Psychrophilic β-d-galactosidase from Arthrobacter sp. 32cB is an interesting candidate for industrial use, as it can hydrolyze lactose at rate comparable to mesophilic βDG from Kluyveromyces lactis. Furthermore, it exhibits additional transglycosylation activity, it catalyzes synthesis of GOS and HOS, for example: lactulose and alkyl glycosides. The functional dimer of ArthβDG has two independent active sites. Each of them is located on the top of TIM-barrel Domain 3 and is constituted of residues from both subunits of the dimer.

The question of the effect of point mutation of the other catalytic residue, E517, has not been answered before. The ArthβDG_E517Q exhibited no catalytic activity, whereas activity of mutant ArthβDG_D207A was severely depleted. As expected of the mutation of the catalytic residue, E517 into glutamine caused loss of function of the enzyme. Mutation of catalytic residue E517 into glutamine resulted in the elevation of the melting temperature of the mutant in respect to ArthβDG by 3.5–5 °C, depending on the investigated buffer solution. In the case of 50 mM sodium phosphate pH 6.0, it attained 49 °C, which means that it was higher by 4.5 °C compared to wild-type protein. The structures of ArthβDG mutants: ArthβDG_D207A and ArthβDG_E517Q, were solved proving that the point mutations within the active site of ArthβDG have no destabilizing effect on protein’s structure. In the case of ArthβDG_E517Q, only a slight change in character of the active site was observed —similar to previously studied loss of function mutant ArthβDG_E441Q. The inactive mutant E517Q was designed specially to enable binding of transglycosylation product—lactulose, in the active site of enzyme and thus elucidating the mode of its binding.

> MSVETPSALADSSPHTAPGSAGRSLELGAADIQDLESFEAGRGALPARAYLQSDAPRLSLNGEWQFRLSPGSRVAPDDGWQLGEALNGFESLPVPSSWPMHGHGAPAYTNVQFPFAVEPPHVPEANPIGDHLVVFEAGPEFFPHALLRFDGIESAGTVWLNGVELGTTRGSRLAHEFDVSGILEQGENTLAVRVAQFSAASYVEDQDMWWLPGIFRDVTLQARPAAGIDDVFVHAGYDHITGEGILKVEASRGGQAIDAVVRVPELALELAAGTEVRVPAVEPWSAEVPKLYEAAVSAAGESVALQIGFRSIAIEDAQFKVNGRRILLRGVNRHEHHPRLGRVVPRDVVEAELRLMKQHNINAIRTSHYPPHPQFLALADQLGFYVVLECDLETHGFESAGWAQNPSDDPQWEDALVDRMRRTVERDKNHASVVMWSLGNEAGTGRNLAAMSRWTKDRDPSRPIHYEGDWSSEHVDVYSRMYASQAETALIGQGIEPALNDAALDARRRAMPFVLCQYVHAMGNGPGGMSEYQALFEKYPRLMGGFVWEWLEHGITVSTADGVDHYGYGGDFGEEVHDGNFVTDGLVDADRRPRPGLLDFKKVIEPLRIDVARDWTGFTLRNGQDFADTSAFSFRYEVEADGGALDGGTVDVAPVAPQSETVVELPGSVAALAAGLSDGRPAVLTVRAVLGADSAWADAGHEVAWGQSVREPGAPVPPAPVEPVQVQDSELTLGPVVFSRATGMPTSIGGVPVEKLGLTLWWAPTDNDLGREWGGADERPLATQWKDAGLNRLHTRLLGISANPGQDGGETLTVRTRVSAADKQYGVLVDYTWSTDGETVGLRTQVRRDGTWVNRGFEVEWARIGLEFVLGEETELVSWFGQGPHQSYPDTGQGARAGWFSLPLAKMDVEYVRPQECGARSGSRSAALQLGGRTLEICGDPFALTVRPYSQDVLDAAAHRPDLKADGRTYLYVDHALRGVGTAACGPGVLEQYRLKPRDADFILTLKVRS> MSRLIFEHQRRLTPPTTRKGTITIEPPPQLPRVVPPSLLRRVLPFLIVILIVGMIVALFATGMRLISPTMLFFPFVLLLAATALYRGGDNKMRTEEVDAERADYLRYLSVVRDNVRAHAAEQRA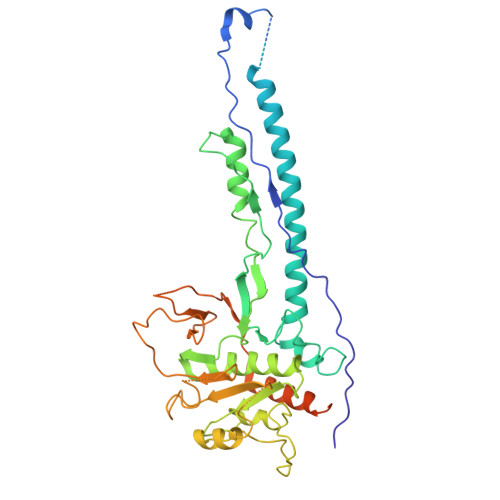ALEWSHPEPEVLATIPGTRRQWERDPRDRDFLVLRAGRHDVPLDAALKVKDTADEIDLEPVAHSALRGLLDVQRTVRDAPTGLDVAKLARITVIGEADEARAAIRAWIAQAVTWHDPTMLGVALAAPDLESGDWSWLKWLPHVDVPNEADGVGPARYLTTSTAELRERLAPALADRPLFPAESGAALKHLLVVLDDPDADPDDIARKPGLTGVTVIHRTTELPNREQYPDPERPILRVADGRIERWQVGGWQPCVDVADAMSAAEAAHIARRLSRWDSNPGYIRSTSTGSATFTTLLGIPDASALDVHLGGIKAFHHHHHHHHHH> MGSLVR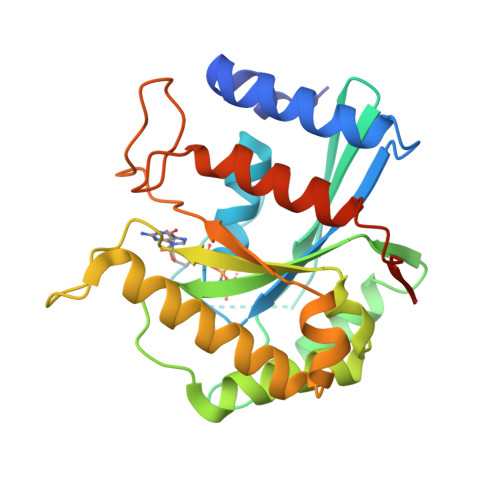EWVGFQQFPAATQEKLIEFFGKLKQKDMNSMTVLVLGKGGVGKSSTVNSLIGEQVVRVSPFQAEGLRPVMVSRTMGGFTINIIDTPGLVEAGYVNHQALELIKGFLVNRTIDVLLYVDRLDVYRVDELDKQVVIAITQTFGKEIWCKTLLVLTHAQFSPPDELSYETFSSKRSDELLKTIRAGSKMRKQEFEDSAIAVVYAENSGRCSKNDKDEKALPNGEAWIPNLVKAITDVATNQRKAIHVDAAALEHHHHHH>[2x]MANDANGRPAPGSRGRGRRPAEEVRAEVLHAVGELLLTEGTAQLTFERVARVSGVSKTTLYKWWPSKGALALDGYFHAVEDTLAFPDTGDVRADLLAQLRAFTHVMTRTPGGRILTEL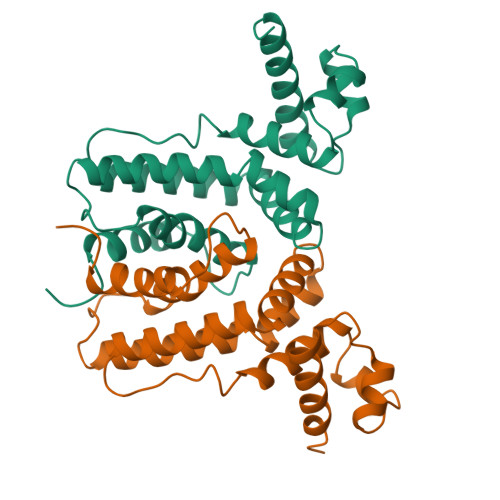IGAAQTDADLATAYRQLYSAQRRALAAERLRHARELGQIRPDVDVQVLVDQLWGAVYHRLLIPDEPVDDAFVTALVTNLLDGVCPRPALEHHHHHH>MDL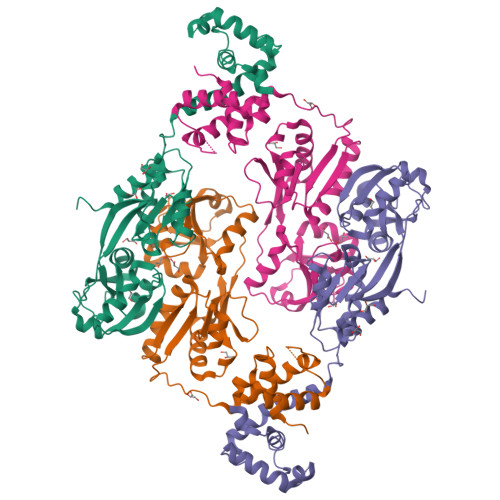RDIDLNLLVVFNQLLLDRSVSTAGEKLGLTQPAVSNSLKRLRTALNDDLFLRTSKGMEPTPYALHLAEPVIYALNTLQTALTTRDSFDPFASTRTFNLAMTDIGEMYFMPPLMEALAQRAPHIQISTLRPNAGNLKEDMESGAVDLALGLLPELQTGFFQRRLFRHRYVCMFRKDHPSAKSPMSLKQFSELEHVGVVALNTGHGEVDGLLERAGIKRRMRLVVPHFIAIGPILHSTDLIATVPQRFAVRCEVPFGLTTSPHPAKLPDIAINLFWHAKYNRDPGNMWLRQLFVELFSEARHHHHHH[2x]> MTYKIGVVGDKDSVSPFRLFGFDVQHGTTKTEIRKTIDEMAKNEYGVIYITEQCANLVPETIERYKGQLTPAIILIPSHQG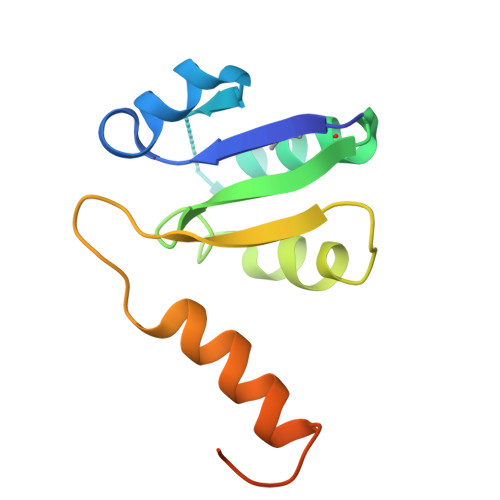TLGIGLEEIQNSVEKAVGQNILSGPSSGENLYFQ>MPHFTVTKVEDPEEGAAASISQEPSLADIKARIQDSDEPDLSQNDITGEHSQLLDDGHKKARNAYLNNSNYEEGDEYFDKNLALFEEEMDTRPKVSSLLNRMANYTNLTQGAKEHEEAENITEGKKKPTKTPQMGTFMGVYLPCLQNIFGVILFLRLTWVVGTAGVLQAFAIVLICCCCTMLTAISMSAIATNGVVPAGGSYFMISRALGPEFGGAVGLCFYLGTTFAAAMYILGAIEIFLVYIVPRAAIFHSDDALKESAAMLNNMRVYGTAFLVLMVLVVFIGVRYVNKFASLFLACVIVSILAIYAGAIKSSFAPPHFPVCMLGNRTLSSRHIDVCSKTKEINNMTVPSKLWGFFCNSSQFFNATCDEYFVHNNVTSIQGIPGLASGIITENLWSNYLPKGEIIEKPSAKSSDVLGSLNHEYVLVDITTSFTLLVGIFFPSVTGIMAGSNRSGDLKDAQKSIPIGTILAILTTSFVYLSNVVLFGACIEGVVLRDKFGDAVKGNLVVGTLSWPSPWVIVIGSFFSTCGAGLQSLTGAPRLLQAIAKDNIIPFLRVFGHSKANGEPTWALLLTAAIAELGILIASLDLVAPILSMFFLMCYLFVNLACALQTLLRTPNWRPRFRYYHWALSFMGMSICLALMFISSWYYAIVAMVIAGMIYKYIEYQGAEKEWGDGIRGLSLSAARFALLRLEEGPPHTKNWRPQLLVLLKLDEDLHVKHPRLLTFASQLKAGKGLTIVGSVIVGNFLENYGEALAAEQTIKHLMEAEKVKGFCQLVVAAKLREGISHLIQSCGLGGMKHNTVVMGWPNGWRQSEDARAWKTFIGTVRVTTAAHLALLVAKNISFFPSNVEQFSEGNIDVWWIVHDGGMLMLLPFLLKQHKVWRKCSIRIFTVAQLEDNSIQMKKDLATFLYHLRIEAEVEVVEMHDSDISAYTYERDLMMEQRSQMLRHMRLSKTERDREAQLVKDRNSMLRLTSIGSDEDEETETYQEKVHMDWTKDKYMASRGQKAKSMEGFQDLLNMRPDQSNVRRMHTAVKLNEVIVNKSHEAKLVLLNMPGPPRNPEGDENYMEFLEVLTEGLERVLLVRGGGSEVITIYS[2x]

Potassium‐coupled chloride transporters (KCCs) play crucial roles in regulating cell volume and intracellular chloride concentration. They are characteristically inhibited under isotonic conditions via phospho‐regulatory sites located within the cytoplasmic termini. Decreased inhibitory phosphorylation in response to hypotonic cell swelling stimulates transport activity, and dysfunction of this regulatory process has been associated with various human diseases. Here, we present cryo‐EM structures of human KCC3b and KCC1, revealing structural determinants for phospho‐regulation in both N‐ and C‐termini.

To understand the structural basis of phospho‐regulation in potassium‐coupled chloride transporters, we used single‐particle cryo‐electron microscopy to study the full‐length wild‐type KCC3b transporter and mutants of this transporter in which two canonical threonines (T940 and T997) and a third KCC3‐specific phosphorylation site (S45), which was shown to play a role for full activation in response to swelling (Melo et␣al, 2013), were replaced. A unique feature observed in the phospho‐mimetic KCC3b‐PM structure is the presence of pronounced density for a short stretch of the otherwise unstructured N‐terminus, a domain that has not been resolved in any of the previously published CCC structures. Electrostatic surface representations of KCC3b in absence or presence of the N‐terminus illustrate that this segment is wedged between CTD and TMD and partially inserted into the inward‐open vestibule created by the helical arrangement of TM2, TM7 and the helices TM1a and TM6b of the transporter core domain. The direct contact with the ion coordinating helices TM1a and TM6b results in a visible obstruction of the ion access path from the intracellular side, suggesting that this domain arrangement could play a role in controlling transport activity. The change in α7 positioning involves a 21° outward movement of the N‐terminal end of α7, accompanied by a conformational change in the β6/α7 loop. By contrast, no densities for ATP or ADP are visible in the map of KCC3b‐PM, which could be the result of small sequence differences in KCC3b.>IAELPPKVSVFVPPRDGFFGNPRKSKLICQATGFSPRQIQVSWLREGKQVGSGVTTDQVQAEAKESGPTTYKVTSTLTIKESDWLGQSMFTCRVDHRGLTFQQNASSMCVPDQDTAIRVFAIPPSFASIFLTKSTKLTCLVTDLTTYDSVTISWTRQNGEAVKTHTNISESHPNATFSAVGEASICEDDWNSGERFTCTVTHTDLPSPLKQTISRPKGVALHRPDVYLLPPAREQLNLRESATITCLVTGFSPADVFVQWMQRGQPLSPEKYVTSAPMPEPQAPGRYFAHSILTVSEEEWNTGETYTCVVAHEALPNRVTERTVDKSTGKPTLYNVSLVMSDTAGTCY[10x];> RILPEVKVEGELGGSVTIKCPLPEMHVRIYLCREMAGSGTCGTVVSTTNFIKAEYKGRVTLKQYPRKNLFLVEVTQLTESDSGVYACGAGMNTDRGKTQKVTLNVHSEYEPSWEEQPMPETPKWFHLPYLFQMPAYASSSKFVTRVTTPAQRGKVPPVHHSSPTTQITHRPRVSRASSVAGDKPRTFLPSTTASKISALEGLLKPQTPSYNHHTRLHRQRALDYGSQSGREGQG;> MKNHLLFWGVLAVFIKAVHVKAQEDERIVLVDNKCKCARITSRIIRSSEDPNEDIVERNIRIIVPLNNRENISDPTSPLRTRFVYHLSDLCKKCDPTEVELDNQIVTATQSNICDEDSATETCYTYDRNKCYTAVVPLVYGGETKMVETALTPDACYPD

FcμR is the IgM antibody isotype-specific Fc receptor involved in the survival and activation of B cells. In this study, we image a complex of the ectodomain of human FcμR and the IgM-Fc pentameric core using single-particle cryogenic electron microscopy (cryo-EM). The analysis reveals multiple binding sites for the N-terminal Ig domain of FcμR on the Cμ4 domain dimers within the IgM constant region and provides a framework for understanding FcμR’s role in immunoglobulin recognition and signalling. A key common feature of the FcμR binding sites is that only the Cμ4 domains are involved in the interactions.

Two binding sites (position 1f and 3f) which have highest occupancies of FcμR, reached high-resolution (3.5 Å and 3.1 Å) in the cryo-EM maps, thus allowing the atomic model interpretation of the FcμR Ig-like domain and the IgM binding interface. Due to the quasi six-fold symmetry within the Cμ4 domains in IgM pentamer, the FcμR molecules at position 1f and 3f share almost identical interactions with the two Cμ4 domains (Cμ4-A and Cμ4-B) in subunits Fcμ1 and Fcμ3 respectively. The Cμ4-B chain of the IgM subunit (grey in Fig. 4b) contains a central hub of residues (Asn465-Glu468) for FcμR binding, which interacts with all three CDR loops on FcμR including CDR1 (Arg45), CDR2 (Thr60/Ser63/Thr65) and CDR3 (Thr110/Asp111). CDR2 of FcμR forms additional interactions including Lys69, which form a hydrogen bond with Glu526 on Cμ4-B chain and Asn66, which contacts neighbouring Cμ4-A chain (Gln510 and Arg514). In addition to the common features, different interactions between FcμR and binding sites at subunits Fcμ1 and Fcμ3 result from the asymmetrical structure of IgM pentamer. The same residue Arg112 in FcμR at position 1f, on the other hand, interacts with Thr571 and Thr574 at the tailpiece in subunit Fcμ5 (chain B) extended from the other side of the IgM-Fc core. Met108 in FcμR also forms hydrogen bonds with Tyr576 at the end of the same tailpiece. The interactions with the tailpiece residues may provide extra stabilisation for FcμR, directly reflected in the high occupancy at position 1f. Interestingly, FcμR at position 1f on IgM, although overlapping with the binding site for pIgR-D1, does not interact with the J chain as pIgR-D1 does when binding to either IgM or IgA, consistent with FcμR binding at other sites where it cannot interact with the J chain.> GAGTDRSATQVVSDMRVGWNIGNSLDSFGQSYNFPYTSLNETYWGNPATTKALIDEVAKAGFNTIRIPVSWGQYTSGSDYQIPDFVMNRVKEVVDYCIVNDMYVILNSHHDINSDYCFYVPNNANKDRSEKYFKSIWTQIAKEFRNYDYHLVFETMNEPRLVGHGEEWWFPRNNPSNDIREAVACINDYNQVALDAIRATGGNNATRCVMVPGYDASIEGCMTDGFKMPNDTASGRLILSVHAYIPYYFALASDTYVTRFDDNLKYDIDSFFNDLNSKFLSRNIP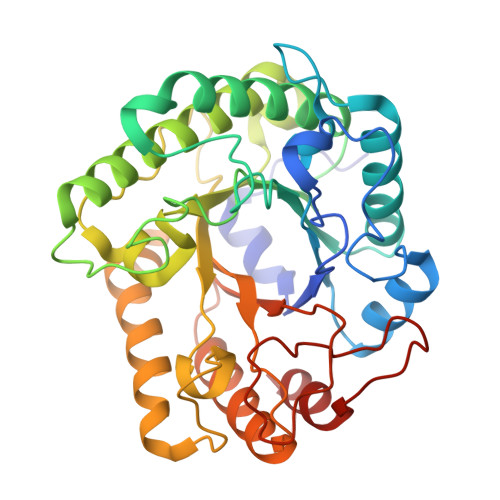VVVGETSATNRNNTAERVKWADYYWGRAARYSNVAMVLWDNNIYQNNSAGSDGECHMYIDRNSLQWKDPEIISTIMKH> MSENIPLRVQFKRMKAAEWARSDVILLESEIGFETDTGFARAGDGHNRFSDLGYISPLDYNLLTNKPNIDGLATKVETAQKLQQKADKETVYTKAESKQELDKKLNLKGGVMTGQLKFKPAATVAYSSS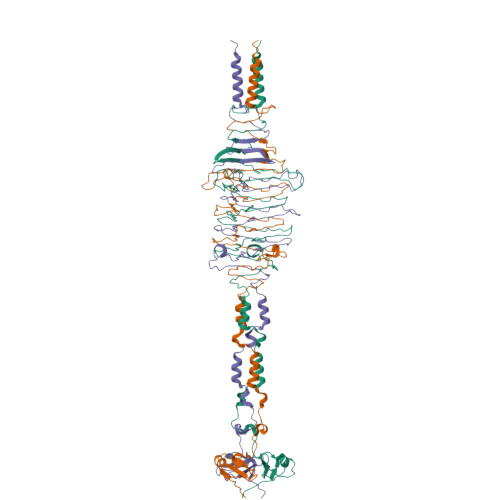TGGAVNIDLSSTRGAGVVVYSDNDTSDGPLMSLRTGKETFNQSALFVDYKGTTNAVNIAMRQPTTPNFSSALNITSGNENGSAMQLRGSEKALGTLKITHENPSIGADYDKNAAALSIDIVKKTNGAGTAAQGIYINSTSGTTGKLLRIRNLSDDKFYVKSDGGFYAKETSQIDGNLKLKDPTANDHAATKAYVDKAISELKKLILKKH The Na+/H+ antiporters are widely distributed secondary active transporters that use the proton motive force to efflux intracellular sodium ions. Mrp antiporters are unique as they usually consist of seven subunits (MrpABCDEFG) encoded in a single operon. Because of the operon’s distinctive properties, Mrp antiporters have been classified in a separate category, cation:proton antiporter-3 (CPA3), in the transporter classification system. They support intracellular pH homeostasis and Na+ efflux in alkali- and halophilic microorganisms and are essential for their survival in challenging environments. The largest two Mrp subunits, MrpA and MrpD, are homologous to each other, have 14 conserved trans-membrane (TM) helices, and are thought to participate in proton translocation.

Therefore we purified the complex in a milder detergent Lauryl Maltose Neopentyl Glycol (LMNG) and collected a dataset again at 35° tilt. The best dimer class refined to 3.7 Å resolution, while the best pseudo-monomer (after symmetry expansion) class refined to 3.0 Å with excellent density in all areas including previously disordered edges. Each monomer consists of seven subunits with a total MW of 213 kDa and comprising 50 TM helices. A striking feature of the Mrp complex is the tightly intertwined interface between the two monomers. The thinness of the dimer interface is mainly due to the two very short N-terminal TMHs of MrpE, of only about 15 residues each, which form the bulk of the interface, resulting in only ~20 Å total protein span across the membrane. A very thin hydrophobic belt is clearly unfavourable for membrane protein folding and so it must have a functional role in Mrp, most likely by acting to significantly disturb and thin a lipid membrane in this area. Our cryo-EM maps revealed strong cation density (stronger than waters) both in DDM and LMNG samples. The cations are coordinated by the conserved H37c and H40c within the two large hydrophilic cavities (which we will call double cavity) surrounding these residues. On the basis of these considerations and according to the analysis of cavities and tunnels by MOLE we propose that the Na+ pathway (which applies also to K+) starts near H42g/H131e, passes by the highly conserved D35f, traverses the large Na+ cavity between MrpF and MrpAC, passes by the key E706a and enters the double cavity where at least two cations, as we observe, can be coordinated between E706a, H37c, H40c and E137d.

>[2x]MLKKNETFYTYCSYKKEDGYVRRGLIVLPTLHIAMFAPFLLALLVPFFYKCIRSLHVGWFVFPLPIALFVYFLSYIDDVRNDEVIRATMPWIPSLRISFDAYVDGLSLLFALLITGIGSLVVLYSIYYLQKGKEPLGNFYVYLLLFMGAMLGVVLSDHLIALYMFWELTSISSFLLIAYWFKRDRSRYGAQKSMLITMFGGLLMLGGFVALAIAGGTYNIRELVHTPLTEHPLFIPALVLILFGAFTKSAQFPFYIWLPDAMEAPTPVSAYLHSATMVKAGIYVIARLTPIFAVSSVWVWTVALVGLVTLCWASFLASKQTDLKAILAYSTVSQLGLITSLLGIGGLSFHYDGMGENVFMVAVLAAIFHLFNHATFKGSLFMVVGIVDHETGTRDIRRLGGLMTIMPITFTIALIGSLSMAGLPPFNGFLSKEMFFTAMLRAKDVAGWAVILPVVAWVASIFTFLYSALLVSRTFFGTYKPHVLKKEAHEAPFGMLIAPIVLASLVVFIGFVPNVLSDSVLAPAVYAVLYGLFAPNEALDVHISHWHGFTPELFMTIGVLLFGLVLYRTFPKWKKIYYRLSERMSLNFFYDQSFVWMERGARSFISRVMNGSMRTYLMYIFTSLVALLLFTIGWHEQWHIDLSRLAHVRVYEVVLAIGILAATVTTVIAKSRLTAIVSLGAVGYAVALFFVLFRAPDLALTQLVIETISVALFLLCFYHLPKFTQKQESVRFHLGNALVSLAVGMTMSIIAFLAYAGKHFDSISQYYVDNTYEKAAGKNMVNVILVDFRGFDTLFEICVLAIAALGIYAMVKLRLAKEEER;>MKRNDVILRTTTAVVTPIIVLFSVQLFFAGHYYPGGGFIGGLMTAGAIVLLLLAFDIETVRKMVPINYKWLVAIGLLFAVGTGMSSMFLDRPFLTHAYKYVHLPLLDHTSLHTAVLFDLGVYFVVVGVTMIIIETIGESD[2x];>[2x]MELLMIVVIGCLFAAATYLLLSKSLLRIIIGTGLLSHGAHLLLLTMGGLKAGAPPLLGEKASRYVDPLPQALILTAIVISFGVTAFFLVLAYRSYQEIGTDHMEGMKGD;>[2x]MSNLLLLPIVIPLVTAIVLIFFPKHVFWQRVVSLAATVGLVVASGALLHRVHTDGIQTLNVGNWPAPFGITLVSDSLSALLVLTTSIIALACLVYSFYAIGHKRETFYYYSFFQFLIVGVNGAFTTGDLFNLFVFFEVMLMSSYVLLVLGGTKIQLRETIKYTLVNVISSALFVVAVAYLYAVTGTLNMAHLADRINALGSSPILTVIAVLFIIVFGLKGAIFPLYFWLPGAYYAPPTPVLALFGGLLTKVGVYSILRTFTLLFTHDAAYTHTLLAWLALGTIIIGVIGAVAYNDMRYIVIYNIIAAVGVMIFGISIMTPESVEGTIFYLLQDMVMKAMLFLFVGIIFSITRSNDIRSFSGLITSYPLLGWAFFIAALSLAGIPPLSGFIGKLLIVKASFDAQLIFEAIVILLSSLLVLYSVMKIFMNGFWGEKKGFEQKQVDGRLFPVLFLLVLSVAYGIGIEFVRPFVLDAVNVLVDPSMYIEAVLKE;>MAFQILLNVILAFVWMFLTVSFDGASFLVGYMIGLFILFILRRFFHSRFYLVPVFVIIKLLFIFFKELILSNIAVAKVVMQRSLTIQPAIFALPTELKKEWEITVLAMLITLTPGTLVLDVSDDGSTLYIHALNSPDVHEAIESIKQSFEKTIMEVSK[2x];>[2x]MMLNIALVILSLAMVGFLYRVVKGPSTADRIIALDAMGITLAGIVAIVSMLLNTSAFLDVILLIGILAFVGTVAFAKFLEKGVVIERGNDR;>MSSNVGTIANALVVVLILLGAVLTLLSAVGAIRLPDVYTRSHAISKSTTLGIMCILLGAFLHFFIENNHFNSRLLLGIVFIFMTSPVAAHLISRAAYYANVERWEGTVRDDLKQKAGGK[2x]> MAGKEKLPKMRLPTRSDMICGYACLKGTAAMRNTKRGSWYIEALAQVFSERACDMHVADMLVKVNALIKDREGYAPGTEFHRCKEMSEYCSTLCRHLYLFPGHPPTAAALE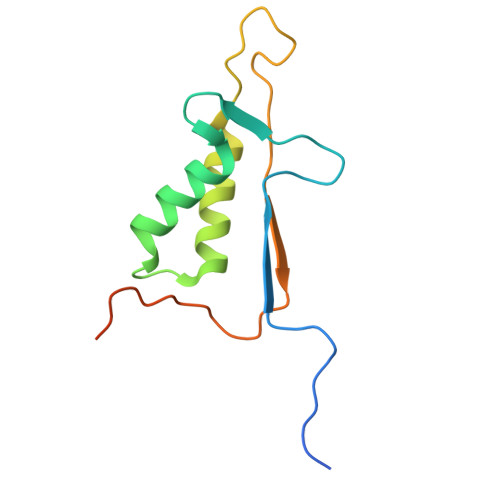HHHHHH> MAVRPGLWPALLGIVLAAWLRGSGAQQSATVANPVPGANPDLLPHFLVEPEDVYIVKNKPVLLVCKAVPATQIFFKCNGEWVRQVDHVIERSTDGSNG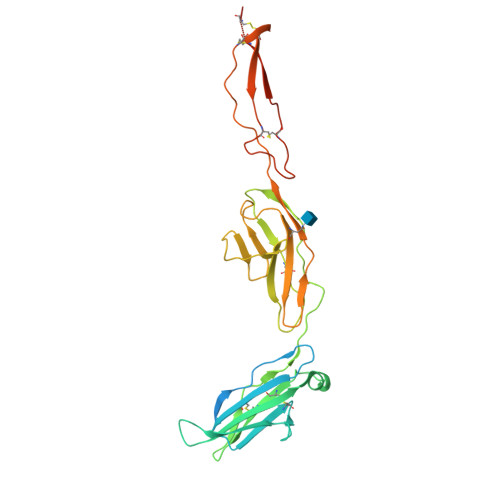LPTMEVRINVSRQQVEKVFGLEEYWCQCVAWSSSGTTKSQKAYIRIAYLRKNFEQEPLAKEVSLEQGIVLPCRPPEGIPPAEVEWLRNEDLVDPSLDPNVYITREHSLVVRQARLADTANYTCVAKNIVARRRSASAAVIVYVDGSWSPWSKWSACGLDCTHWRSRECSDPAPRNGGEECQGTDLDTRNCTSDLCVHTASGPEDV>PPGPPGPPGPPGPPAPPGP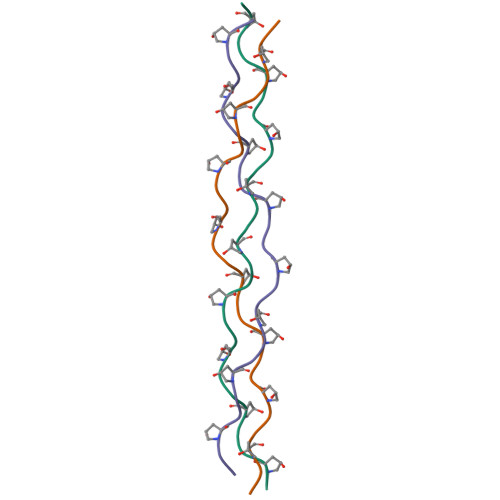PGPPGPPGPPG[3x]5,5'-pentane-1,5-diylbis(1,3,4-thiadiazol-2-amine) | C9 H14 N6 S2 | 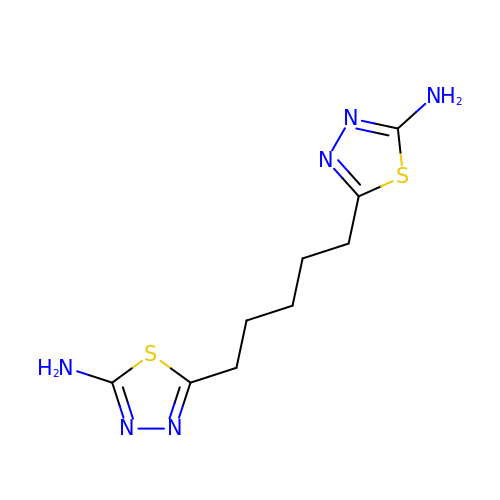KEOUOMDZUGENOX-UHFFFAOYSA-N>[2x]MELRVGNRYRLGNKIGSGSFGDIYLGTDIAAGEEVAIKLECVKTKHPQLHIESKIYKMMQGGVGIPTIRWCGAEGDYNVM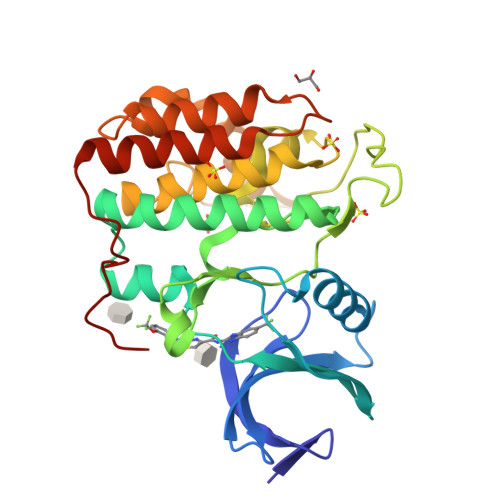VMELLGPSLEDLFNFCSRKFSLKTVLLLADQMISRIEYIHSKNFIHRDVKPDNFLMGLGKKGNLVYIIDFGLAKKYRDARTHQHIPYRENKNLTGTARYASINTHLGIEQSRRDDLESLGYVLMYFNLGSLPWQGLKAATKRQKYERISEKKMSTPIEVLCKGYPSEFATYLNFCRSLRFDDKPDYSYLRQLFRNLFHRQGFSYDYVFDWNMLKF> MQNIPPQVQAMLGQLDTYQQQLQLVIQQKQKVQADLNE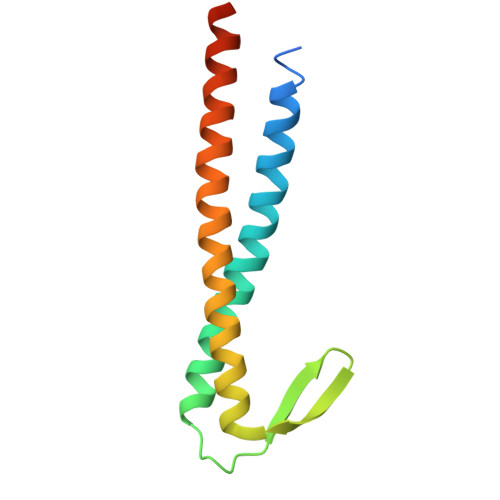AKKALEEIETLPDDAQIYKTVGTLIVKTTKEKAVQELKEKIETLEVRLNALNRQEQKINEKVKELTQKIQAALRPPTAG> GSVPATLPQLTPTLVSLLEVIEPEVLYAGYDSSVPD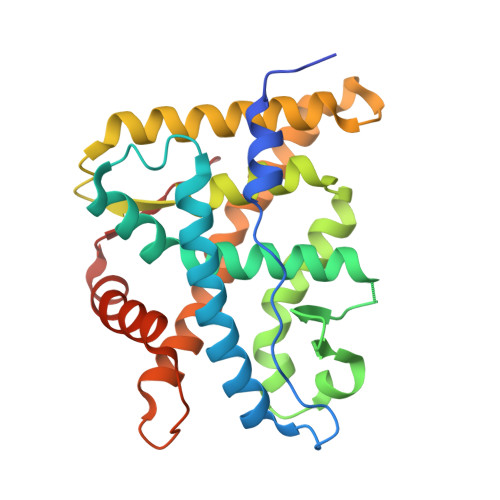STWRIMTTLNMLGGRQVIAAVKWAKAIPGFRNLHLDDQMTLLQYSWMYLMAFALGWRSYRQSSANLLCFAPDLIINEQRMTLPGMYDQCKHMLYVSSELHRLQVSYEEYLCMKTLLLLSSVPKDGLKSQELFDEIRMTYIKELGKAIVKREGNSSQNWQRFYQLTKLLDSMHEVVENLLNYCFQTFLDKTMSIEFPEMLAEIITNQIPKYSNGNIKKLLFHQK>MPATHHSSATSAERPTVVGRIPVLDVRPVVQRGRRPAKAVTGESFEVSATVFREGHDAVGANVVLRDPRGRPGPWTPMRELAPGTDRWGATVTAGETGTWSYTVEAWGDPVTTWRHHARIKIPAGLDTDLVLEEGARLYERAAADVPGREDRRELLAAVDALRDESRPAASRLAAALTPQVDAVLARHPLRDLVTSSDPLPLLVERERALYGAWYEFFPRSEGTPHTPHGTFRTAARRLPAIAAMGFDVVYLPPIHPIGTTHRKGRNNTLSATGDDVGSPWAIGSPEGGHDSIHPALGTLDDFDHFVTEAGKLGLEIALDFALQCSPDHPWVHKHPEWFHHRPDGTIAHAENPPKKYQDIYPIAFDADPDGLATETVRILRHWMDHGVRIFRVDNPHTKPVAFWERVIADINGTDPDVIFLAEAFTRPAMMATLAQIGFQQSYTYFTWRNTKQELTEYLTELSGEAASYMRPNFFANTPDILHAYLQHGGRPAFEVRAVLAATLSPTWGIYSGYELCENTPLREGSEEYLDS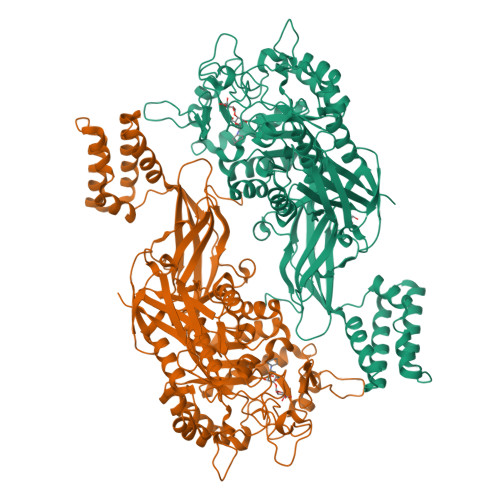EKYQLKPRDWTRAAREGTTIAPLVTRLNTIRRENPALRQLRDLHFHPTDKEEVIAYSKRQGSNTVLVVVNLDPRHTQEATVSLDMPQLGLDWHESVPVRDELTGETYHWGRANYVRLEPGRTPAHVCTVLRPSHPQIGGSHTTALHHHHHH[2x]> SNASFDETSKRNEGRVKNIVYLNFDGTITGAHGKEVISSPLCEALSTKATFDERMRYKNEYDASDNKIKITENAKNFLQDVNKLHPQVKIVIISRNHENYIKALLEFENIDHRNIIIYPRGVGNTIGPGEDKYKAVVSHEEKPECLPGFRLICDDD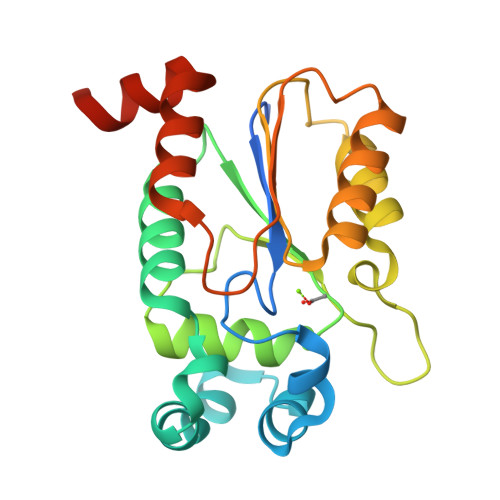EVDGEEMCNGLIHTGRSQLVKFHNEKPGQFKWGEYFKEILTNCDIAVKEYLNGKIGSRFH> SGSSEQELAAIVRDLGCGPYFLGTHDKRFPGFLAGNKLACAIVNTAGRETGGVHWLAFGWNPRSRTCYMFDPFGFSDRRLKQIYSFEYEAMLRRSALALSPDRCLSLEQSTQTVQGPDSAACGLFCCMFLHAFVHWPDRPMDGNPTMNLLTGVPNGMLQSPQVLPTLRRNQEKLYRFLAHHSPYFRSHRAAIEHATAFD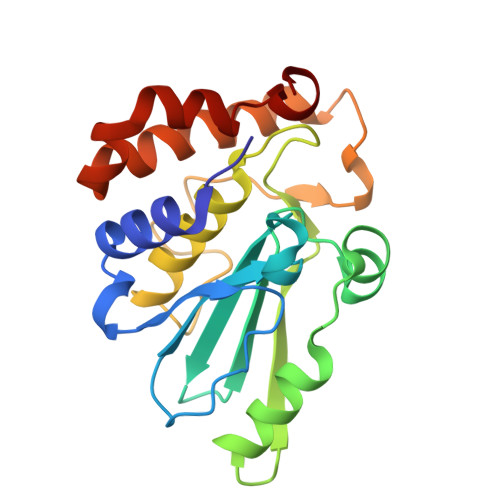KMKQL>MSIPVTEFRQFSEQQPAFRVLKPWWDVFTDYLSVAMLMIGVFGCTLQVMQDKIICLPKRVQPAQNHSSVPNVSQAVISTTPLPPPKPSPTNPATVEMKGLKTDLDLQQYSFINQMCYERALHWYAKYFPYLVLIHTLVFMLCSNFWFKFPGSSSKIEHFISILGKCFDSPWTTRALSEVSGEDSEEKDNRKNNMNRSGTIQSGPEGNLVRSQSLKSIPEKFVVDKSAAGALDKKEGEQAKALFEKVKKFRLHVEEGDILYAMYVRQTVLKVIKFLIIIAYNSALVSKVQFTVDCNVDIQDMTGYKNFSCNHTMAHLFSKLSFCYLCFVSIYGLTCLYTLYWLFYRSLREYSFEYVRQETGIDDIPDVKNDFAFMLHMIDQYDPLYSKRFAVFLSEVSENKLKQLNLNNEWTPDKLRQKLQTNAHNRLELPLIMLSGLPDTVFEITELQSLKLEIIKNVMIPATIAQLDNLQELCLHQCSVKIHSAALSFLKENLKVLSVKFDDMRELPPWMYGLRNLEELYLVGSLSHDISKNVTLESLRDLKSLKILSIKSNVSKIPQAVVDVSS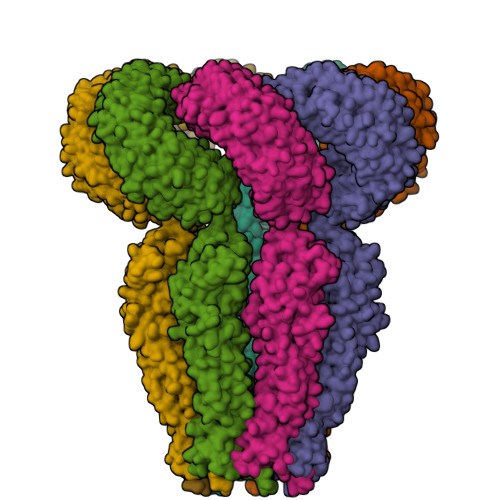HLQKMCVHNDGTKLVMLNNLKKMTNLTELELVHCDLERIPHAVFSLLSLQELDLKENNLKSIEEIVSFQHLRKLTVLKLWYNSIAYIPEHIKKLTSLERLFFSHNKVEVLPSHLFLCNKIRYLDLSYNDIRFIPPEIGVLQSLQYFSITCNKVESLPDELYFCKKLKTLKIGKNSLSVLSPKIGNLLFLSYLDIKGNHFEVLPPELGDCRALKRARLVVEDALFETLPSDVREQMKADALEVLFQ[7x]> MKKEVRKVRIALASPEKIRSWSYGEVEKPETINYRTLKPERDGLFDERIFGPIKDYECACGKYKRQRFEGKVCERCGVEVTRSIVRRYRMGHIELATPAAHIWFVKDVPSKIGTLLDLFATELEQVLYFNKYIVLDPKGAVLDGVPVEKRQLLTDXXXXXXXXXXXXXXXXXXXXXXXXXXXXXXXXXXXXIDARMGAEAIQELLKELDLEKLERELLEEMKHPSRARRAKARKRLEVVRAFLDSGNRPEWMILEAVPVLPPDLRPMVQVDGGRFATSDLNDLYRRLINRNNRLKKLLAQGAPEIIIRNEKRMLQEAVDAVIDNGRRGSPVTNPGSERPLRSLTDILSGKQGRFRQNLLGKRVDYSGRSVIVVGPQLKLHQCGLPKRMALELFKPFLLKKMEEKAFAPNVKAARRMLERQRDIKDEVWDALEEVIHGKVVLLNRAPTLHRLGIQAFQPVLVEGQSIQLHPLVCEAFNADFDGDQMAVHVPLSSFAQAEARIQMLSAHNLLSP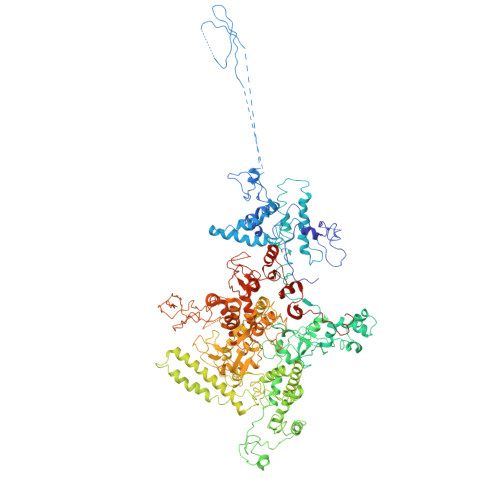ASGEPLAKPSRDIILGLYYITQVRKEKKGAGMAFATPEEALAAYERGEVALNAPIVVAGRETSVGRLKFVFANPDEALLAVAHGLLDLQDTVTTRYLGRRLETNPGRILFARIVGEAVGDEKVAQELIQMDVPQEKNSLKDLVYQAFLRLGMEKTARLLDALKYYGFTLSTTSGIITIGIDDAVIPEEKQRYLEEADRKLRQIEQAYEMGFLTDRERYDQVIQLWTETTEKVTQAVFNNFEENYPFNPLYVMAQSGARGNPQQIRQLCGMRGLMQKPSGETFEVPVRSSFREGLTVLEYFISSHGARKGGADTALRTADSGYLTRKLVDVAHEIVVREADCGTTKYISVPLFQMDEVTRTLRLRKRSDIESGLYGRVLAREVEALGRRLEEGRYLSLEDVHFLIKAAEAGEVREVPVRSPLTCQTRYGVCQKCYGYDLSMARPVSIGEAVGVVAAESIGEPGTQLTMRTFHTGGVAVGTDITQGLPRVIELFEARRPKAKAVISEIDGVVRIEEGEDRLSVFVESEGFSKEYKLPKDARLLVKDGDYVEAGQPLTRGAIDPHQLLEAKGPEAVERYLVDEIQKVYRAQGVKLHDKHIEIVVRQMLKYVEVTDPGDSPLLEGQVLEKWDVEALNERLIAEGKVPVAWKPLLMGVTKSALSTKSWLSAASFQNTTHVLTEAAIAGKKDELIGLKENVILGRLIPAGTGSDFVRFTQVVDQRTLKAIEEARKEAVEAKEKEAPRRPVRREQPGKGL(1S)-1,4-anhydro-1-(5-carbamoyl-4-hydroxy-1H-pyrazol-3-yl)-5-O-phosphono-D-ribitol 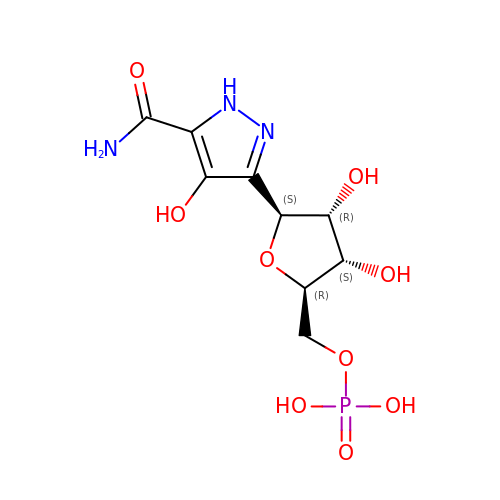| C9 H14 N3 O9 P | CUHDHRMGDRLFLH-FLLFQEBCSA-N LEA was engineered to represent the evolutionary node that acquired the unique ability to photoconvert from the ancestral green fluorescent protein (ALL-GFP), which was engineered on the basis of ancestral gene reconstruction from the great star coral Montastraea cavernosa. Perhaps the most important mutation to make LEA photoconvertible is modifying the chromophore to a His-Tyr-Gly (HYG) chromophore, making it a Kaede-type FP. Another green-to-red pcFP named the least-evolved ancestor (LEA) was also discovered to display pronounced photoswitching of both the green and red forms. Several photoconversion mechanisms have been proposed for the Kaede-like pcFPs, and most mechanisms involve a β-elimination reaction and backbone breakage to extend the conjugation between Gly64 and His62 that forms the red chromophore, although the complete photocycle remains largely unanswered.

To round out the set of related FPs, a new FP with a novel chromophore via ncAA incorporation is presented as LEA-H62X, wherein X = 3-methyl-histidine. A rather surprising finding is that the 3-methyl-histidine (3 mH)-bearing chromophore in LEA-H62X leads to pronounced on→off photoswitching (orange), where the GB absorption peak exhibits a large intensity decrease after 2 hours of 505 nm illumination, significantly more than LEA, together with a large increase in the GA’ population. The ncAA incorporation of an extra methyl group to the chromophore histidine ring greatly reduces the photoconversion efficiency versus LEA and the LEA-A69T mutant, but surprisingly enhances the dynamic photoswitching under 505 nm irradiation which can result in a larger red yield and red:green contrast under dual illumination than traditional 400 nm irradiation of LEA-H62X. LEA-A69T crystallized in space group P212121 with a full tetramer in the asymmetric unit, while LEA-H62X crystallized in I222 with a single protomer per asymmetric unit; both crystal forms were described previously for LEA. However, the local environment surrounding the P-ring of LEA and LEA-H62X are essentially indistinguishable; therefore, the blueshifted absorption of LEA-H62X likely stems from the slightly twisted structure that results in a reduced conjugation between the P- and I-rings, consistent with the blueshift according to the particle-in-a-box principle. Regarding the drastic change to the photoswitching behavior under 505 nm irradiation, the pre-twisted P-ring of LEA-H62X may enable the substantially more efficient on→off photoswitching than LEA. The extra methyl group causes the largest horizontal shift of the imidazole ring in LEA-H62X relative to LEA, with LEA-A69T lying between them. The distance between Glu211 and the α -carbon comprising the bridge between the I-ring and His62 is 3.7 Å in LEA-H62X versus 3.5 Å in LEA.

> MSVIKSDMKIKLRMEGTVNGHKFVIEGEGEGKPYEGTQTMNLKVKEGAPLPFAYDILTTVFXNRVFAKYPKHIPDYFKQSFPEGYSWERSMTFEDGGICTARNDITLEGDCFFNEIRFDGVNFPPNGPVMQKKTLKWEPSTEKMYVRDGVLTGDINMALLLEGGGHYRCDFKTTYKAKKGVQLPDYHFVDHCIEILSHDKDYNNVKLYEHAVAHSGLPRQAKHHHHHH>[2x]MVEKRVFEMPHFTTFGGKQIKNVKVGWEAYGTLNDAKSNVILITHYFSGSSHAAGKYDENDPAPGYWDSIIGPGKAIDTDRFYVISVDTLANLNAYDPHVITTGPTSINPDTGKPYGLDFPVVTIRDFVNVQKALLESLGISKLYAVIGPSMGSM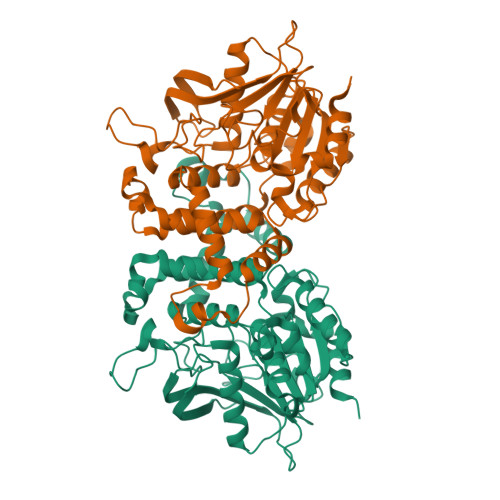QAIDWASAYPGWVERMISVIGAGQSDAWTTAALEHWATPITLDKNWNNGAYSKEQAPLNGLAASLMLITQNALTPSFFNQTGNTLGYKNVESAPLNDIRQSHSIVNWLRERAKTRAKSMDANHLLYLVRACQLFVAGHQGNLEQGLASIKAKTLFIPAQTDLLLMPYLSQSAHQGLTSMNNDSTLVTLNGKLGHDEGVTNVSAQAQAIRQFLEND The kink-turn (k-turn) is a widespread helical junction in RNA. The standard k-turn comprises a duplex RNA containing a three-nucleotide bulge followed by tandem G:A and A:G base pairs. The G:A base pairs adopt trans sugar-Hoogsteen conformation, also known as sheared base pairs, and the overall structure is tightly kinked, with an included angle between the axes of the flanking helices of 50°. In the absence of metal ions or binding proteins, the RNA adopts a conformation that is not tightly kinked, but rather bent in the manner of a simple three-nucleotide bulge. Many (but not all, see below) k-turns adopt the k-turn conformation on addition of divalent metal ions, but some will not.

The RAGATH-18 RNA was crystallized as a duplex containing two k-turns with two-fold symmetry. The RNA forms a standard k-turn structure, where both the tandem G:A base pairs at the 1b:1n and 2n:2b positions form the usual trans-sugar-Hoogsteen pairs. The standard cross-strand hydrogen bonds from the L1 O2′ to A1n N1, and from the -1n O2′ to A2b are formed. The latter is accepted by A2b N3, and further stabilized by a hydrogen bond between G-1n N2 and A2b O2′. Thus the RNA adopts the N3 conformation as predicted. The A3b:G3n base pair is also a standard trans-sugar-Hoogsteen pair, and the G4b:U4n adopts a cis-wobble base pair conformation with two hydrogen bonds between the nucleobases. Examination of the RAGATH-18 crystal structure now reveals unassigned electron density in the major groove. In addition to Fo− Fc density close to the terminal phosphates, we observe three peaks in the planes of successive base pairs, close to the Hoogsteen edges of G2n, G3n and to the O4 and O6 atoms of U4n and G4b respectively. U4n O4 is prominent in the major groove because of the wobble conformation of the base pair. This local conformation may stabilize a chain of bound metal ions, providing a plausible explanation for the enhanced folding of k-turns with 4b:4n = G:U.

>[6x]GUCUAUGAAGGCUGGAGAC> MTNKDNPKFHTISTEYIDYLREADSKVPFNKDEQHSRPYVGVLEKINGHDYF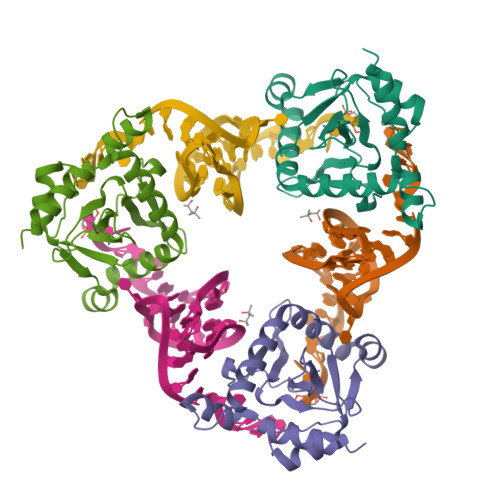VPLTSRNDKNFNSQVSVKLFDNDEKRIGVLLVNNMIPVPEKECKEIDIAEKTAADPQYGNLMLKQYLFLKENMDRVTNKVEKVYKDVTVQGKPSHKQKFLKGVCCDFPKLEEKCQEYKERDQAKERDKARRIAYMRQMGRER> GAMATTKIRIFVPATNSPELRWELTLFALDVIRSPSAAESMKVGAAFTLISMYSERPGALIRSLLNDPDIEAVIIDVGSMVNGIPVMERRGDKAQEEMEGLMRILKTARDSSKGKTPFVDSRAYGLRITDMSTLVSAVITIEAQIWILIAKAVTAPDTAEESETRRWAKYVQQKRVNPFFALTQQWLTEMRNLLSQSLSVRKFMVEILIEVKKGGSAKGRAVEIISDIGNYVEETGMAGFFATIRF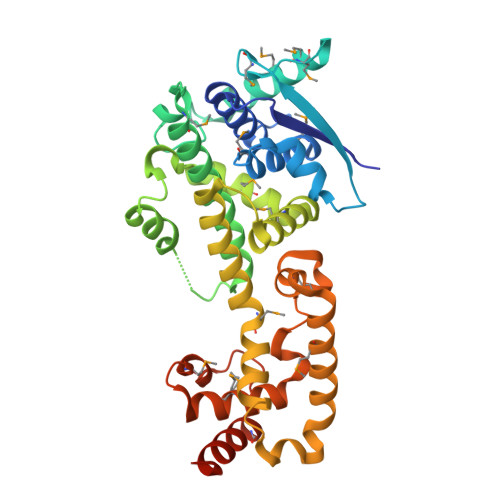GLETRYPALALNEFQSDLNTIKSLMLLYREIGPRAPYMVLLEESIQTKFAPGGYPLLWSFAMGVATTIDRSMGALNINRGYLEPMYFRLGQKSARHHAGGIDQNMANRLG Atypical protein kinase C (aPKC) is a key apical-basal polarity determinant and Par complex component. The atypical protein kinase C (aPKC in Drosophila or PKCι/PKCζ isozymes in mammals), its binding partner Par6, and the small guanosine triphosphatase Cdc42 are three essential determinants of apical membrane identity in both Drosophila and mammals (Fletcher et al., 2012, Harris and Tepass, 2008, Hutterer et al., 2004, Izumi et al., 1998, Joberty et al., 2000, Lin et al., 2000, Wodarz et al., 2000). aPKC isoforms PKCι and PKCζ have regulatory regions distinct from those of other PKC isozymes, but share a conserved catalytic protein kinase domain. Like many protein kinases, activation of aPKC requires activation-loop phosphorylation and an αC-helix conformation compatible with Lys-Glu salt-bridge formation to bind ATP and serve to align residues within the R spine (Kornev et al., 2008).

To explore and capture a substrate peptide bound to PKCιKD-2P, we used an artificial substrate (FKRQGSVRRR, referred to hereafter as F-X-Rshort peptide). This efficient PKCι substrate closely resembles the aPKC consensus motif identified from screening randomly oriented peptide libraries by Cantley and co-workers (Nishikawa et al., 1997). We therefore determined a crystal structure for F-X-Rshort bound to PKCιKD-2P in the presence of Mn-ADP and AlF3, a transition-state analog. Manganese ions corresponding to Mg1 and Mg2 ions are present in the structure, and the AlF3 is positioned as expected to mimic the transition state for the γ-phosphate. Surprisingly, the structure revealed that the F-X-R motif at F−5 and R−3 engages precisely the same site 1 residue contacts (M341PKCι, M344PKCι and L381PKCι, and D339PKCι) as the F−9 and R−7 contacts used by Par3CR3, despite their different position in the primary sequence. Moreover, the R−3 side chain directly makes a hydrogen bond with the ribose hydroxyl, perhaps sensing nucleotide occupancy. We also observe an R+2 side-chain bridging contact between phospho-T412PKCι and G398PKCι main-chain carbonyl, making two key hydrogen bonds with these groups. We note that many aPKC substrates have an R+2 side chain, suggesting that direct contact with a phosphorylated activation loop may reflect a common interaction made by aPKC substrates. From the Par3CR3 structure, it is evident that the F-X-Rshort peptide does not inhibit PKCι because it lacks a C-terminal inhibitory motif.

>SLGLQDFDLLRVIGRGSYAKVLLVRLKKTDRIYAMKVVKKELVNDDEDIDWVQTEKHVFEQASNHPFLVGLHSCFQTESRLFFVIEYVNGGDLMFHMQRQRKLPEEHARFYSAEISLALNYLHERGIIYRDLKLDNVLLDSEGHIKLTDYGMCKEGLRPGDTTSTFCGTPNYIAPEILRGEDYGFSVDWWALGVLMFEMMAGRSPFDIVGSSDNPDQNTEDYLFQVILEKQIRIPRSLSVKAASVLKSFLNKDPKERLGCHPQTGFADIQGHPFFRNVDWDMMEQKQVVPPFKPNISGEFGLDNFDSQFTNEPVQLTPDDDDIVRKIDQSEFEGFEYINPLLMSAEECV[2x];>[2x]ERMRPFKRQGSVRRRV> SNSGTEQQNPRGSSLLTDPESITKSDPYNPNISLLISGEVFTNFRNLIKRVNFRKATTLNGKRISDTFDINS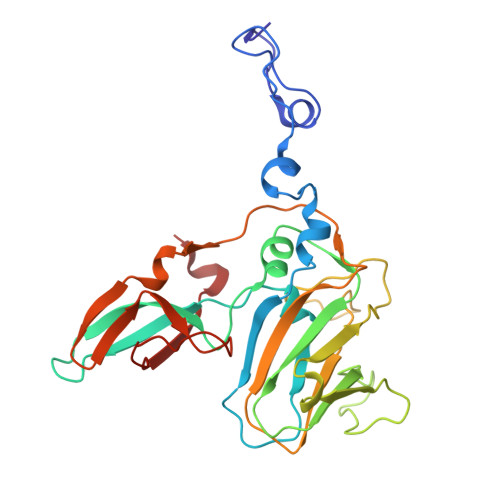LIEAPRLDIAQYVDTETKEAKYGFSYFWSAPTTLNIVAEMYALYRGGVRVKVVTEKGVDFVRATVSPQQTYGSDVAPTTHISTPLAIEQIPIKGVAEFQIPYYAPCLSSSFRANSETFYYSSGRNNLDIATSPPSINRYYAVGAGDDMDFSIFIGTPPCIHASQTAQFTKIKQGKVYDLRYDQYDPFREVQDGTAFLNARSIEDSDLL>MEKRKIILD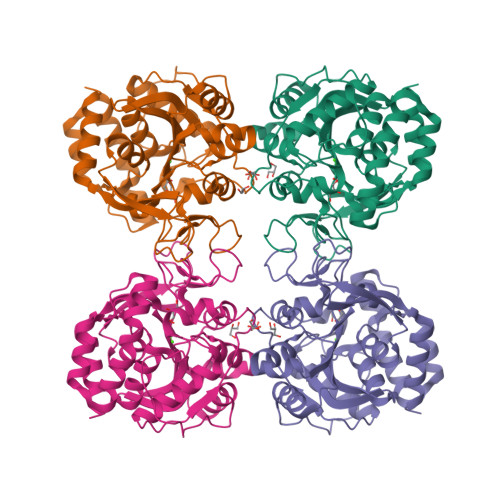CDPGHDDAIAIMMAAKHPAIDLLGITIVAGNQTLDKTLINGLNVCQKLEINVPVYAGMPQPIMRQQIVADNIHGDTGLDGPVFEPLTRQAESTHAVKYIIDTLMASDGDITLVPVGPLSNIAVAMRMQPAILPKIREIVLMGGAYGTGNFTPSAEFNIFADPEAARVVFTSGVPLVMMGLDLTNQTVCTPDVIARMERAGGPAGELFSDIMNFTLKTQFENYGLAGGPVHDATCIGYLINPDGIKTQEMYVEVDVNSGPCYGRTVCDELGVLGKPANTKVGITIDTDWFWGLVEECVRGYIKTH[4x]>[3x]SNADTGWLTMPDNDHAQVRATADKSSTGDVKILLEVQLAPGWKTYWRSPGEGGVAPEINWTQSVSDMIWHWPSPSAFDVAGIHTQGYDKEVVFPIELKSVDSDNLNGVLTLSTCSNVCILTDYSLNLDLNEPAPADFEWQYNQAMAKVPVTSGLISAVSSDYRNSQLTL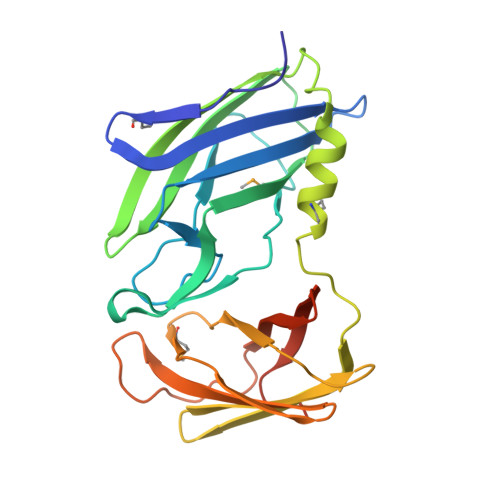SLQREQGDWHQPNIYLDPPQGMLYGIPQLTAKGDHLSVTVDVTDDWGDAAGDITGKALSFVVTDDGYSRQVNDTIGQGDSASLPTADS> MVSVINTVDTSHEDMIHDAQMDYYGTRLATCSSDRSVKIFDVRNGGQILIADLRGHEGPVWQVAWAHPMYGNILASCSYDRKVIIWREENGTWEKSHEHAGHDSSVNSVCWAPHDYGLILACGSSDGAISLLTYTGEGQWEVKKINNAHTIGCNAVSWAPAVVPGSLIDHPSGQKPNYIKRFASGGCDNLIKLWKEEEDGQWKEEQKLEAHSDWVRDVAWAPSIGLPTSTIASCSQDGRVFIWTCDDASSNTWSPKLLHKFNDVVWHVSWSITA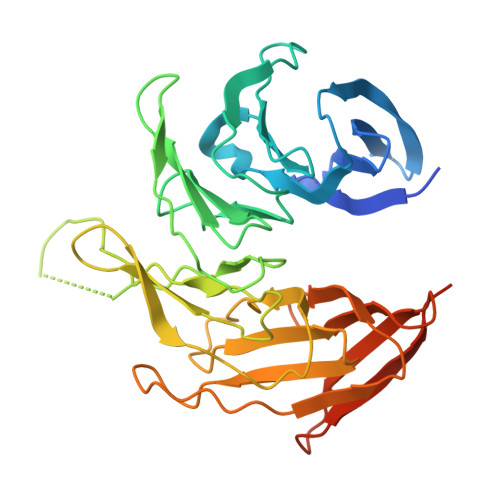NILAVSGGDNKVTLWKESVDGQWVCISDVNKGQGSVSASVTEGQQNEQ Coxsackie virus B5 (CVB5) is a member of Enterovirus-B (EV-B) species, which can cause various human diseases, such as viral encephalitis; herpangina; hand, foot, and mouth disease (HFMD); aseptic meningitis; and acute flaccid paralysis (1–3). Similar to other EV-B species, CVB5 is a nonenveloped, positive-sense single-strand RNA (+ssRNA) virus. P2, and P3 will break down into nonstructural proteins responsible for genome replication, whereas P1 is the precursor form of structural proteins VP1-VP4, which could be packaged into an icosahedral capsid. Here, we determined the atomic structures of CVB5 in three forms: mature full (F) particle (2.73 Å), intermediate altered (A) particle (2.81 Å), and procapsid empty (E) particle (2.95 Å).

In agreement with the results from AUC and EM, after data processing, three distinctive maps corresponding to F, A and E particles were reconstructed and refined to the resolutions of 2.73 Å, 2.81 Å, and 2.95 Å, respectively, according to the Fourier shell correlation at a threshold of 0.143, which allowed an atomic model for the majority of the main chains and sides chains to be manually fitted or built in. Compared with the map of the F particle, both maps of A and E particles had an expansion of ~4% with large openings on the 2-fold axes. Comparing the compact CVB5 F particle with the expanded A particle, we found that the expansion of CVB5 was largely attributable to the tectonic movements of viral proteins, accompanied by a ~5.5° counterclockwise rotation of the protomeric building unit pivoting about the 3-fold axis and a ~7 Å shift away of VP1 and VP3 from the particle center. This movement results in a more elongated structure and broadening of the surface mesa. Furthermore, the whole GH loop of VP3 seems to shift from its position. We noted that the first seven residues of VP1 visualized on A particle would traverse the capsid and stop on the surface of the capsid, which was distinctive from the E particle where the corresponding residues were disordered, and all the other remaining residues were present on the interior of the capsid. Based on the previous studies on enteroviruses, it is reasonable to deduce that with the particle expansion, the GH loop of VP3 moved upward from the quasi-3-fold hole to form the classic β-hairpin structure to obstruct the off-axis channels and aid in the widening of the 2-fold helices (residues 90 to 98) connecting the C and D strands of VP2. This rearrangement likely spared enough room allowing the extension of VP1 N-terminus to pass through the inner surface to reach the 2-fold gate and later slip into the quasi-3-fold hole, reminiscent of what has been proposed in other enteroviruses (i.e. EV71, E30, CVA16, and poliovirus).

> QTRHVKNYHSRSESTVENFLCRSACVFYTTYRNHGTDGDNFGYWVISTRQVAQLRRKLEMFTYARFDLELTFVITSTQEQSTIQGQDSPVLTHQIMYVPPGGPVPTKVNSYSWQTSTNPSVFWTEGSAPPRMSIPFISIGNAYSMFYDGWAKFDKQGTYGINTLNNMGTLYMRHVNDGSPGPIVSTVRIYFKPKHVKTWVPRPPRLCQYQKAGNVNFEPTGVTESRTDITTMQ;> RVRSITLGNSTITTQECANVVVGYGVWPTYLNDDEATAEDQPTQPDVATCRFYTLESVMWQQSSPGWWWKFPDALSNMGLFGQNMQYHYLGRAGYTVHVQCNASKFHQGCLLVVCVPEAEMGCATLANKPDQKSLSNGETANMFESQNSTGQTAVQANVINAGMGVGVGNLTIFPHQWINLRTNNSATIVMPYINSVPMDNMFRHNNFTLMIIPFAPLSYSTGATTYVPITVTVAPMCAEYNGLRLAG;> GLPTMLTPGSNQFLTSDDFQSPSAMPQFDVTPEMDIPGQVNNLMEIAEVDSVVPVNNTEGKVLSIESYQIPVQSNSTNGSQVFGFPLMPGASSVLNRTLLGEILNYYTHWSGSIKLTFMFCGSAMATGKFLLAYSPPGAGAPTTRKEAMLGTHVIWDVGLQSSCVLCIPWISQTHYRYVVVDEYTAGGYITCWYQTNIVVPADTQSDCKILCFVSACNDFSVRMLKDTPFIKQDNFYQ> MVRIFLMALLMASLWIQGSPAPLASANPEELGKVVTAIEQLDQMRIGLASTLEGGTSEPTLDTFKAVCAPVGKQAKEIAAANGWQVRQVALKYRNPNHAPRTALDVQALNQFDNNHHLQAFWQTDKEGVHYFRRID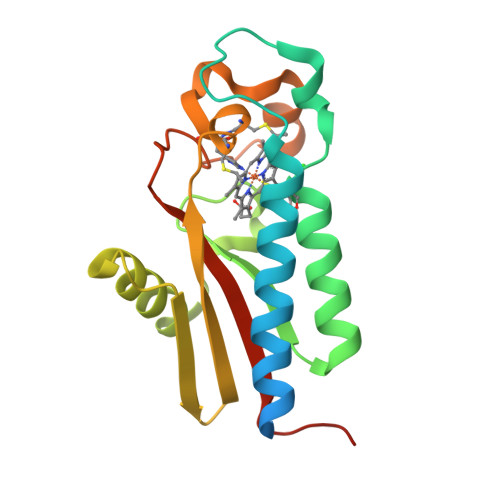VQASCLACHGAKNRRPAFIQEKYPSDRAYGFRVGDLRGMYAVTIPQIQQALQTSP> MERRSLAQELKKWAVEEMGLPAQKAPSEEMLQRLFIGQCGDIWKFIIRHIHSHRTVRKIEGNLLWYQQLQHTEAQRTAEEEQQQRRKQLCKEILELRAELHHLQEQIQTAEREIVGQDLNCERAQDLCRRSLLLRAFNKKREEECEALCQSNKKIQYRCEQLQEIRRA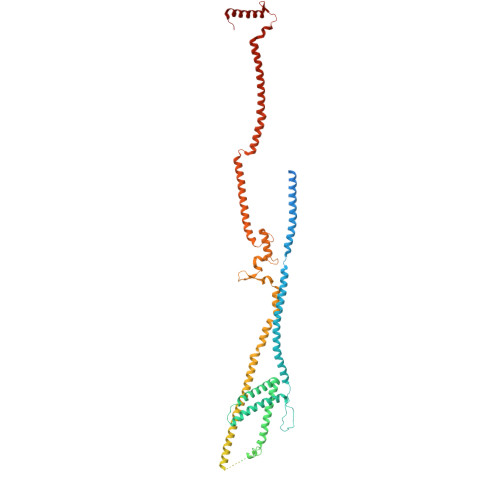SQREVMFSAVDPDLSSSTFLEPEVLRDVREVCKLRFKFLRSLHDDSISSSVHPGKEDLRSLSHQQWMSMAEKVWNTHTPNHILAALERLTLNSTQELKKLQFSQAADLSKGPSCQLKEFSEPITQSRSCNESTHLDPQETLPSFHSLIQEGWANSVKVSSELRRVQSQAQALSEHLAERIQEIHKKLSDGSEVSVLTRAAFDAELRCVILRGCRDALMQECRMLQEEAAGKKQEMKLLQQQQQNIQEACLLLDKKQKHIQILIKGNSSSKSQIRRSSVEAQKYVQDKLLPWPQEIIQESQRLQDSIQKEVKHFSAICLPALLKVSTDGFNLLPSRELSINRMSNTHAPYYGIFKGIYESVRLPLYKAPESVLSHVADMKKQLFFLRSQLSSRSEAISKTQRALQKNTNPDTDALLKSLSDHYSLELDEMVPKMQRLIQQCEKHQEYGKEVQATVMDWWEQPVQLCLPSEERGGLTLRQWRERWTVAVTALQRATGSRS> MVEKEEAGGGISEEEAAQYDRQIRLWGLEAQKRLRASRVLLVGLKGLGAEIAKNLILAGVKGLTMLDHEQVTPEDPGAQFLIRTGSVGRNRAEASLERAQNLNPMVDVKVDTEDIEKKPESFFTQFDAVCLTCCSRDVIVKVDQICHKNSIKFFTGDVFGYHGYTFANLGEHEFVEEKTKVAKVSQGVEDGPDTKRAKLDSSETTMVKKKV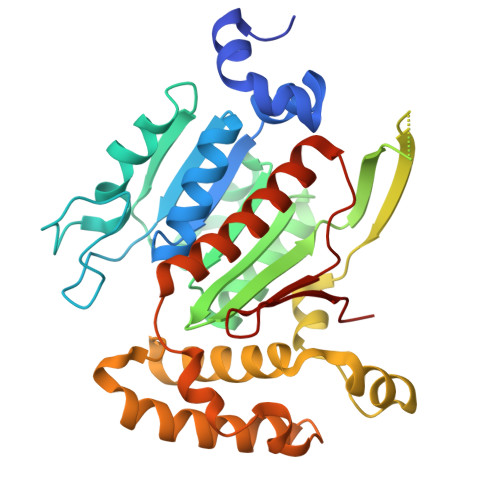VFCPVKEALEVDWSSEKAKAALKRTTSDYFLLQVLLKFRTDKGRDPSSDTYEEDSELLLQIRNDVLDSLGISPDLLPEDFVRYCFSEMAPVCAVVGGILAQEIVKALSQRDPPHNNFFFFDGMKGNGIVECLGPK N-hydroxycyclohex-1-ene-1-carboxamide 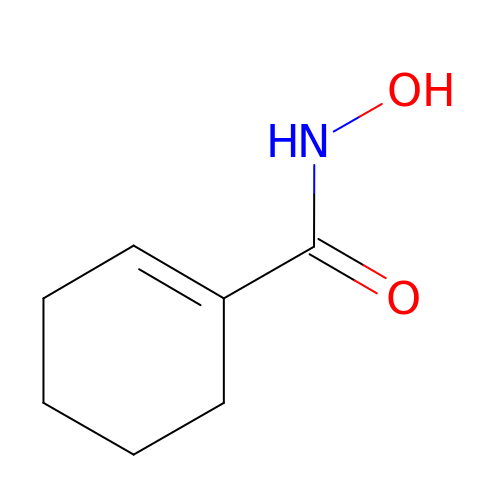| C7 H11 N O2 | NMUKJRPCVOESRU-UHFFFAOYSA-N> GGGGGUGUGCCCGGCAUGGGUGCAGUCUAUAGGGUGAGAGUCCCGAACUGUGAAGGCAGAAGUAACAGUUAGCCUAACGCAAGGGUGUCCGUGGCGACAUGGAAUCUGAAGGAAGCGGACGGCAAACCUUCGGUCUGAGGAACACGAACUUCAUAUGAGGCUAGGUAUCAAUGGAUGAGUUUGCAUAACAAAACAAAGUCCUUUCUGCCAA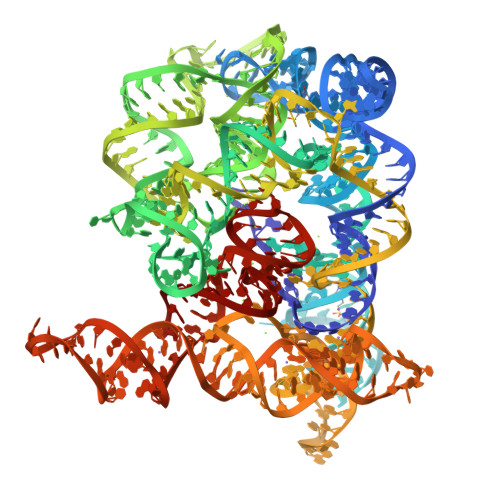AGUUGGUACAGAGUAAAUGAAGCAGAUUGAUGAAGGGAAAGACUGCAUUCUUACCCGGGGAGGUCUGGAAACAGAAGUCAGCAGAAGUCAUAGUACCCUGUUCGCAGGGGAAGGACGGAACAAGUAUGGCGUUCGCGCCUAAGCUUGAACCGCCGUAUACCGAACGGUACGUACGGUGGUGUG>[2x]MVPATIARFSQLNAEDQLALIWFAYLEMGKTLTIAAPGAASMQLAENALKEIQAMGPLQQTQAMCDLANRADTPL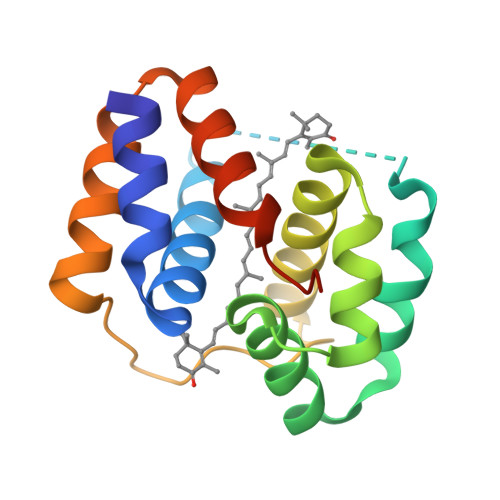CRTYASWSPNIKLGFWYRLGELMEQGFVAPIPAGYQLSANANAVLATIQGLESGQQITVLRNAVVDMGFTAHHHHHH> RPQGATVSLWETVQKWREYRRQCQRSLTEDPPPATDLFCNRTFDEYACWPDGEPGSFVNVSCPWYLPWASSVPQGHVYRFCTAEGLWLQKDN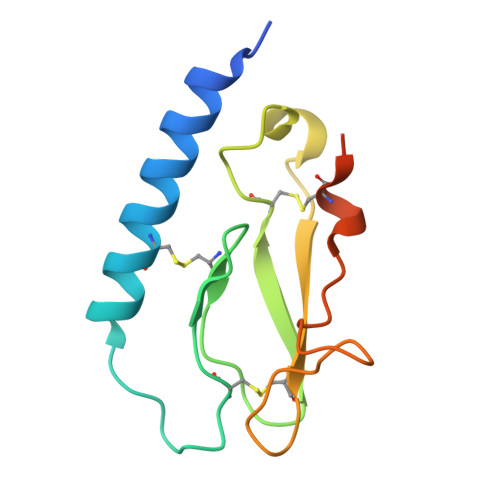SSLPWRDLSECEESKRGERSSPEE The crystal structures and inhibitor complexes of two industrially important ω-aminotransferase enzymes from Pseudomonas aeruginosa and Chromobacterium violaceum have been determined in order to understand the differences in their substrate specificity. The two enzymes share 30% sequence identity and use the same amino acceptor, pyruvate; however, the Pseudomonas enzyme shows activity towards the amino donor β-alanine, whilst the Chromobacterium enzyme does not. Both enzymes show activity towards S-α-methylbenzylamine (MBA), with the Chromobacterium enzyme having a broader substrate range. It appears that the different rigidity of the protein scaffold contributes to the substrate specificity observed for the two ω-­aminotransferases.

Attempts to crystallize C. violaceum Am:PyAT with a small excess of PLP (100 µM) resulted in the structure of the apoenzyme. C. violaceum Am:PyAT elutes with an apparent molecular mass of 100 kDa on a size-exclusion chromatography column, which corresponds to a dimer. This enzyme is found to be a dimer in the crystal, with the asymmetric unit containing one (apoenzyme and mCPP complex) or two (holoenzyme) dimers. Significant structural rearrangements accompany cofactor binding in C. violaceum (CV) Am:PyAT, as also described by Humble et al.. This includes unwinding of the α-helix (residues CV 317–322) to form a loop covering the PLP phosphate group. The N-terminus (up to residue 36), which is disordered in the apoenzyme structure, becomes ordered in the holoenzyme structure and occupies the position of the unwound helix.

>MQKQRTTSQWRELDAAHHLHPFTDTASLNQAGARVMTRGEGVYLWDSEGNKIIDGMAGLWCVNVGYGRKDFAEAARRQMEELPFYNTFFKTTHPAVVELSSLLAEVTPAGFDRVFYTNSGSESVDTMIRMVRRYWDVQGKPEKKTLIGRWNGYHGSTIGGASLGGMKYMHEQGDLPIPGMAHIEQPWWYKHGKDMTPDEFGVVAARWLEEKILEIGADKVAAFVGEPIQGAGGVIVPPATYWPEIERICRKYDVLLVADEVICGFGRTGEWFGHQHFGFQPDLFTAAKGLSSGYLPIGAVFVGKRVAEGLIAGGDFNHGFTYSGHPVCAAVAHANVAALRDEGIVQRVKDDIGPYMQKRWRETFSRFEHVDDVRGVGMVQAFTLVKNKAKRELFPDFGEIGTLCRDIFFRNNLIMRACGDHIVSAPPLVMTRAEVDEMLAVAERCLEEFEQTLKARGLA[2x]>MLLNALASLGHKGIKTLRTFGRAGLMLFNALVGKPEFRKHAPLLVRQLYNVGVLSMLIIVVSGVFIGMVLGLQGYLVLTTYSAETSLGMLVALSLLRELGPVVAALLFAGRAGSALTAEIGLMRATEQLSSMEMMAVDPLRRVISPRFWAGVISLPLLTVIFVAVGIWGGSLVGVSWKGIDSGFFWSAMQNAVDWRMDLVNCLIKSVVFAITVTWISLFNGYDAIPTSAGISRATTRTVVHSSLAVLGLDFVLTALMFGN[2x];>[2x]MEQSVANLVDMRDVSFTRGNRCIFDNISLTVPRGKITAIMGPSGIGKTTLLRLIGGQIAPDHGEILFDGENIPAMSRSRLYTVRKRMSMLFQSGALFTDMNVFDNVAYPLREHTQLPAPLLHSTVMMKLEAVGLRGAAKLMPSELSGGMARRAALARAIALEPDLIMFDQPFVGQDPITMGVLVKLISELNSALGVTCVVVSHDVPEVLSIADHAWILADKKIVAHGSAQALQANPDPRVRQFLDGIADGPVPFRYPAGDYHADLLPGS;>[2x]MSESLSWMQTGDTLALSGELDQDVLLPLWEMREEAVKGITCIDLSRVSRVDTGGLALLLHLIDLAKKQGNNVTLQGVNDKVYTLAKLYNLPADVLPR;>MQTKKNEIWVGIFLLAALLAALFVCLKAANVTSIRTEPTYTLYATFDNIGGLKARSPVSIGGVVV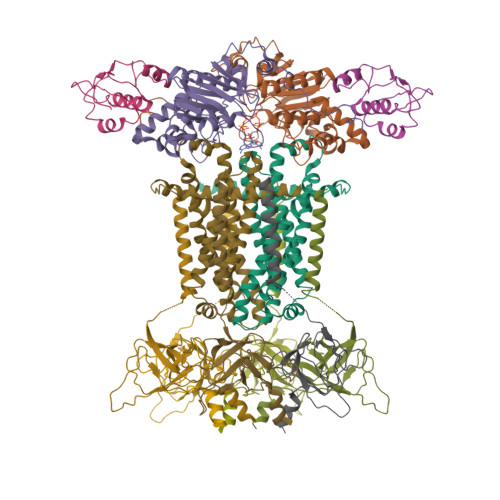GRVADITLDPKTYLPRVTLEIEQRYNHIPDTSSLSIRTSGLLGEQYLALNVGFEDPELGTAILKDGDTIQDTKSAMVLEDLIGQFLYGSKGDDNKNSGDAPAAAPGNNETTEPVGTTK[6x]>IDVKNAHAVVEQTEENVFLIPLKHLRDSQFVGTLLVGVPPQEIHPIFDTGSTNLWVVTTDCEEESCKKVKRYNPYKSKTFRRSFIGKNLHIVFGSGSISGSIGKETFVLGDHTVRNQTFGLVESESNDSLNGDNIFDYIDFEGIVGLGFPEMLSAGKVSFFDNLLSQNKNLSPQFSFYISPEDNTSTFLVGGVSKSFYEGSIYMLPVVKEYYWEVELDGIYVGEKKICCEEKSYAIFDTGTSYNTMPSAQMKGFFDVVPSAPCTEENYQEVLKNYPVIKYLFGDLVIELLPEEYMILNEESCIPAYMQIDVPSEKNHAYLLGSIAFMRHYYTVFVRGAGGQPSMVGVAKARAAAEAAQKVAE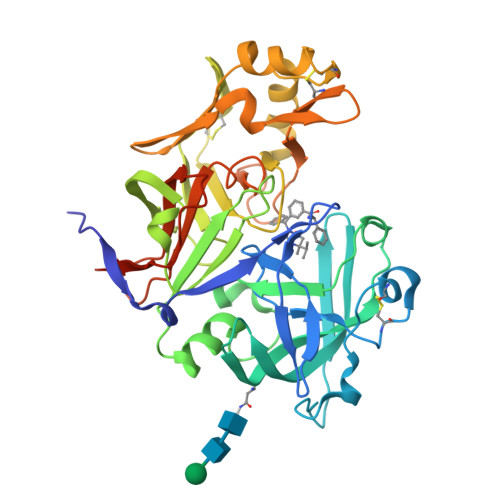LENLYFQGDYKDDDDKH[4x]> GSPIPHHDEKTWNVGSSNRNKAENLLRGKRDGTFLVRESSKQGCYACSVVVDGEVKHCVINKTATGYGFAEP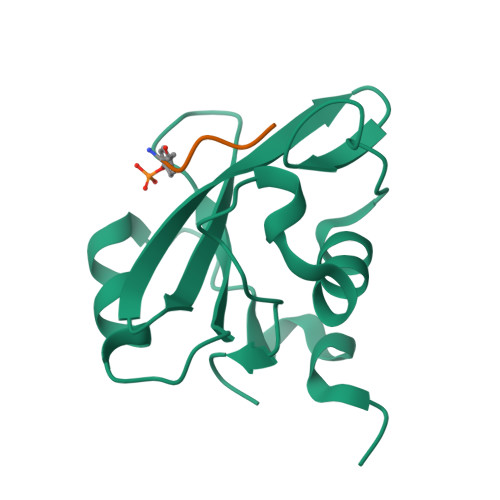YNLYSSLKELVLHYQHTSLVQHNDSLNVTLAYPVYAQQRR;> YVPML> LCEEGLKRLQQMLAEYQAQSDVPQEVCDQILEAAKESSVGEDGVRSQVKIRKPNGKNNIRYEYDLDHIDCKKNEITFYRHINYSDGSKRKIQYTVGIEGFVDIYDFVNVQKCDAQVYDTKTSKTVGGRKIINSEFAGKTVTTKGGDVRFDSDGFPDFTPYSKKTVRVIGLTGDMANDVPL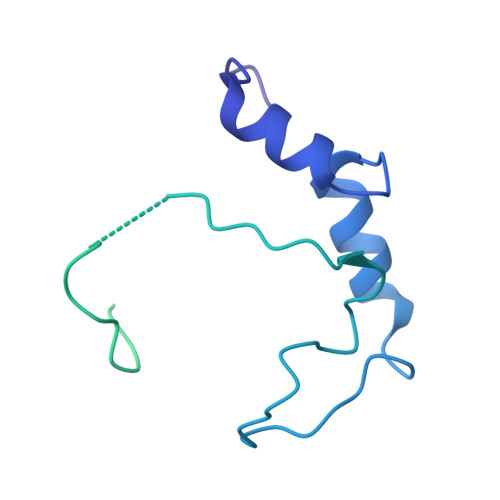AMARAKITKYDKSKYVWHHHQDGKTMMLIPKSVHSVRNGGVAATGGRSVIQHNLLNPNNKLNYSSPEELV> TTTILGFKISMPIMIAPTAMQKMAHPEGEYATARAASAAGTIMTLSSWATSSVEEVASTGPGIRFFQLYVYKDRNVVAQLVRRAERAGFKAIALTVWKDVAWLQTITSLPILVKGVITAEDARLAVQHGAAGIIVSNHGARQLDYVPATIMALEEVVKAAQGRIPVFLDGGVRRGTDVFKALALGAAGVFIGRPVVFSLAA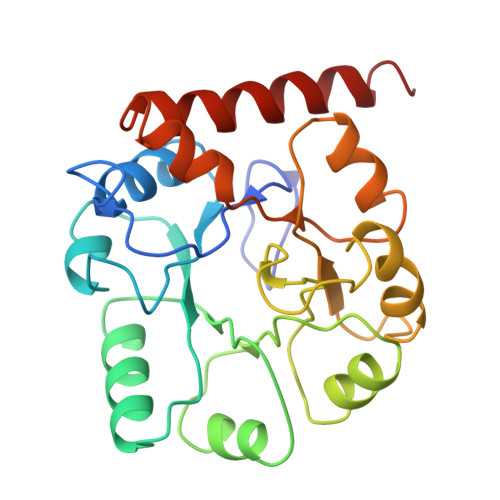EGEAGVKKVLQMMRDEFELTMALSG4-[[(3S)-3-cyclopropyl-2-azaspiro[3.3]heptan-2-yl]methyl]-N-[[(3R)-1-[6-(methylamino)pyrimidin-4-yl]-3-oxidanyl-piperidin-3-yl]methyl]-2-oxidanyl-benzamide 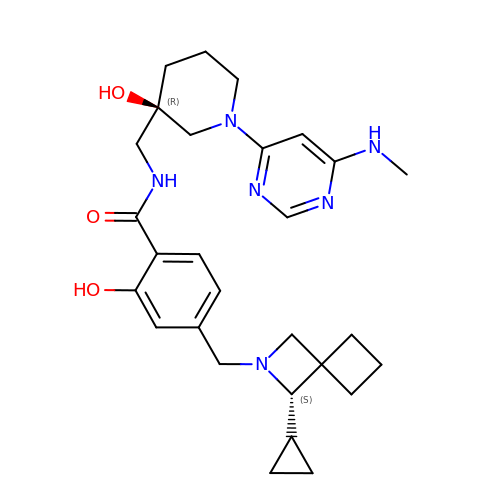| C28 H38 N6 O3 | JWBZACHWPMPYIU-LBNVMWSVSA-N> KPF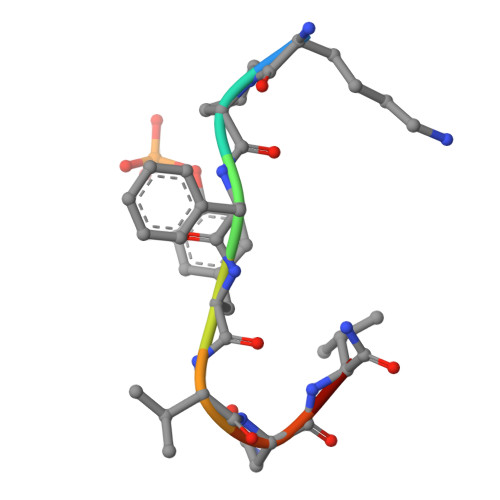YVNVX>MDIWYGTAAVPKDLDNSAVTIGVFDGVHRGHQKLINATVEKAREVGAKAIMVT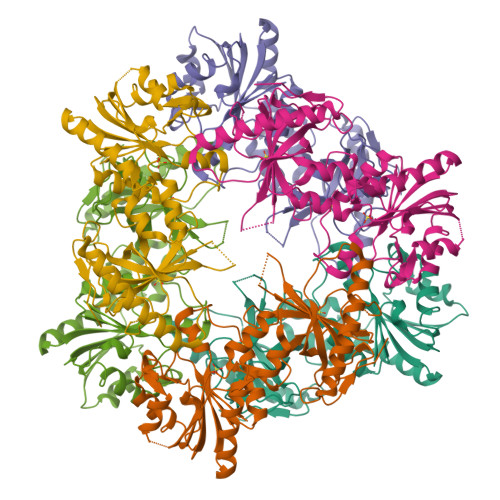FDPHPVSVFLPRRAPLGITTLAERFALAESFGIDGVLVIDFTRELSGTSPEKYVEFLLEDTLHASHVVVGANFTFGENAAGTADSLRQICQSRLTVDVIDLLDDEGVRISSTTVREFLSEGDVARANWALGRHFYVTGPVVRGAGRGGKELGFPTANQYFHDTVALPADGVYAGWLTILPTEAPVSGNMEPEVAYAAAISVGTNPTFGDEQRSVDSFVLDRDADLYGHDVKVEFVDHVRAMEKFDSVEQLLEVMAKDVQKTRTLLAQDVQAHKMAPETYFLQAES[2x]>AVTCGQVASSLAPCIPYARSAGGAVPPACCSGIKTLDGMARTTPDRQATCKCLKSASTSISGINYGLVASLPAKCGVNIPYKISPSTDCARVK[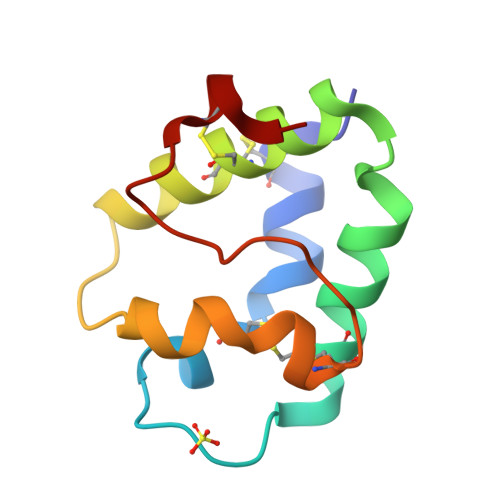4x]>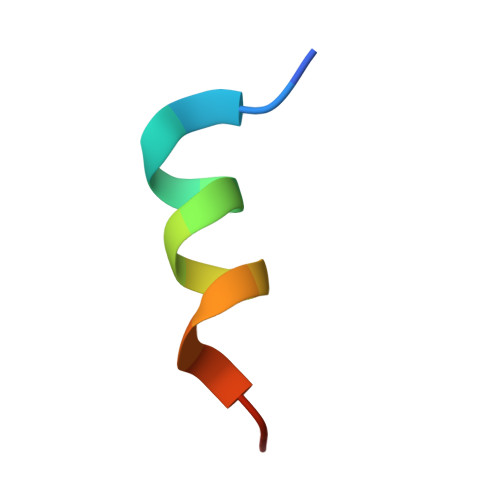 KETAAAKFERQHIDSX>[6x]MESTLGSDLARLVRVWRALIDHR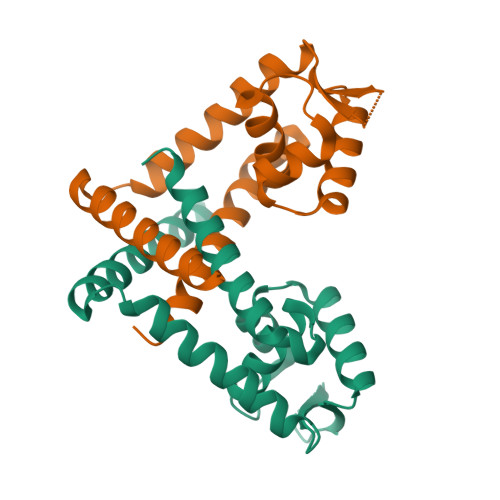LKPLELTQTHWVTLYNINRLPPEQSQIQLAKAIGIEQPSLVRTLDQLEEKGLITRHTSANDRRAKRIKLTEQSSPIIEQVDGVISSTRKEILGGISSDEIAVLSGLIDKLEKNIIQLQTKLEHHHHHH> MIYPIFIFKTVEGFDGYFPDIDGCFFAGNTFADISKNAEEAFAVHIEALMNEGFPLPSPPKDPHRYIDDPRLK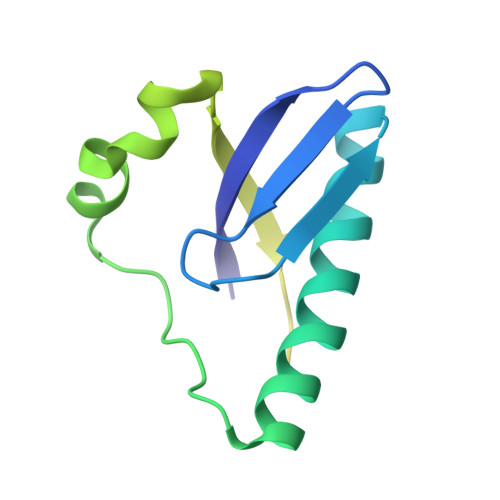EEGGILGFVEIDPAKYESKAVKFNLTMSQNLLTAIDKFIATNRGYKNRSQFLAELAREKIISLEHHHHHH> MFERFTDRARRVVVLAQEEARMLNHNYIGTEHILLGLIHEG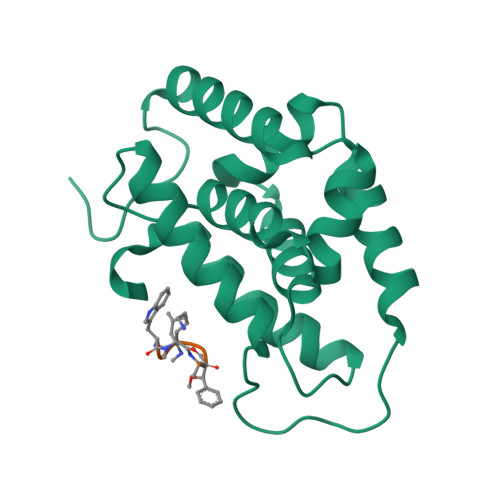EGVAAKSLESLGISLEGVRSQVEEIIGQGQQAPSGHIPFTPRAKKVLELSLREALQLGHNYIGTEHILLGLIREGEGVAAQVLVKLGAELTRVRQQVIQLLSGYQGKLEHHHHHH;> WXAFVLI> MDQECIENYAKVNGIYIYYKLCKAPEEKAKLMTMHGGPGMSHDYLLSLRDMTKEGITVLFYDQFGCGRSEEPDQSKFTIDYGVEEAEALRSKLFGNEKVFLMGSAYGGALALAYAVKYQDHLKGLIVSGGLSSVPLTVKEMNRLIDELPAKYRDAIKKYGSSGSYENPEYQEAVNYFYHQHLLRSEDWPPEVLKSLEYAERRNVYRIMNGPNEFTITGTIKDWDITDKISAIKIPTLITVGEYDEVTPNVARVIHEKIAGSELHVFRDCSHLTMWEDREGYNKLLSDFIL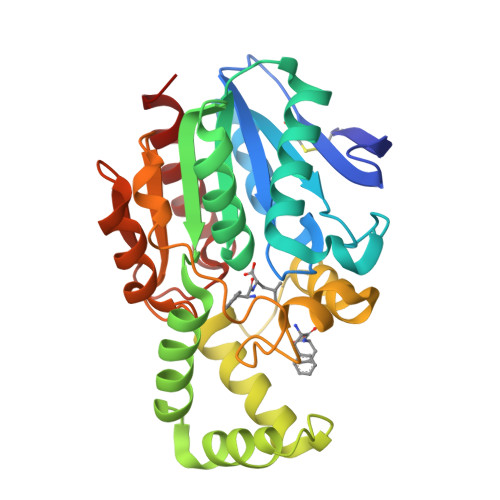KHL> MTFISRFAPDQPRKGADILVEALERQGVETVFAYPGGASMEIHQALTRSSSIRNVLPRHEQGGVFAAEGYARSSGKPGICIATSGPGATNLVSGLADALLDSVPLVAITGQVPRRMIGTDAFQETPIVEVTRSITKHNYLVMDVEDIPRIIEEAFFLATSGRPGPVLVDVPKDIQQQLAIPNWEQAMRLPGYMSRMPKPPEDSHLEQIVRLISESKKPVLYVGGGCLNSSDELGRFVELTGIPVASTLMGLGSYPCDDELSLHMLGMHGTVYANYAVEHSDLLLAFGVRFDDRVTGKLEAFASRAKIVHIDIDSAEIGKNKTPHVSVCGDVKLALQGMNKVLENRAEELKLDFGVWRNELNVQKQKFPLSFKTFGEAIPPQYAIKVLDELTDGKAIISTGVGQHQMWAAQFYNYKKPRQWLSSGGLGAMGFGLPAAIGASVANPDAIVVDIDGDGSFIMNVQELATIRVENLPVKVLLLNNQHL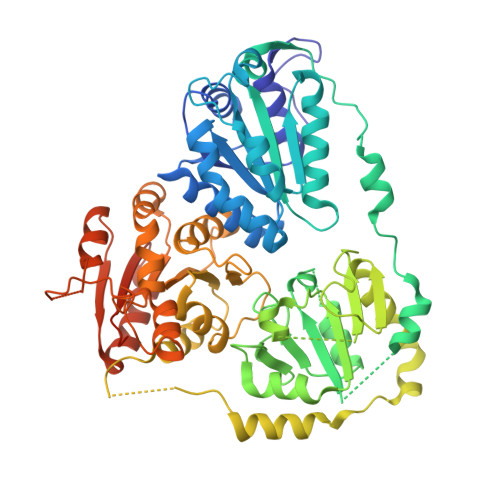GMVMQWEDRFYKANRAHTFLGDPAQEDEIFPNMLLFAAACGIPAARVTKKADLREAIQTMLDTPGPYLLDVICPHQEHVLPMIPSGGTFNDVITEGDGRIKY>[4x]MPGGRGRIGVILPANNAGMEYDLWKMAPEGVSIHSTRMKPTKGCEPENVEEFEKE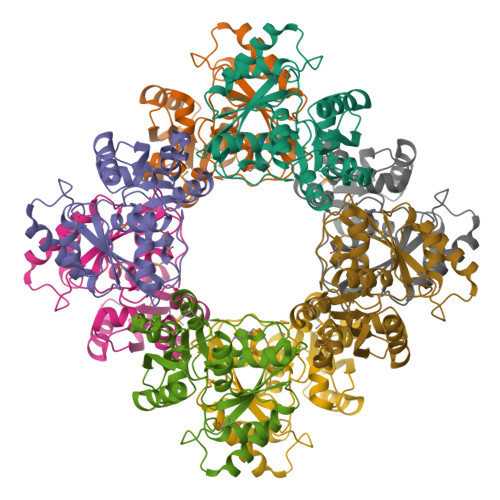LKYSYSLLAEVSDIIIYGRTYGTHKHAHVIKRVIKDVVIPEESVYELLKKLNVRKLWIGTPYIKERTLEEVEWWRNKGFEIVGYDGLGKIRGIDISNTPIFTIYRLVKRHLNEVLKADAVYIACTALSTYEAVQYLHEDLDMPVVSENAAAMWEALNKLKIKAKLPGF>MSQNRQLLYPREEMVSLVRSLDRPQENGLFSQDVLLQYPELAESYTKVCPNRCDLATAADRAAKGAYGYDVQLTTLKEDIRLMVNNCILFNGAEGAYADAARTFEKF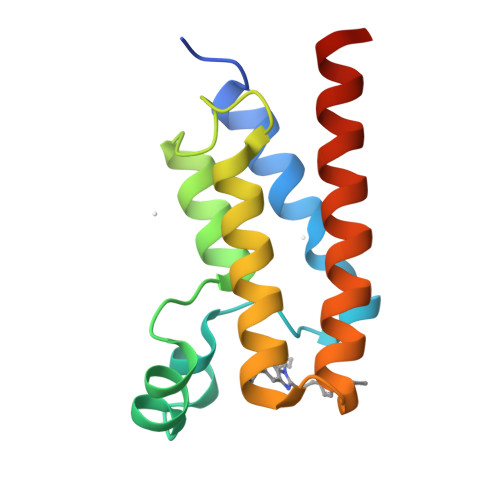AMGKIDAYISQKVGGRRL[4x]>[2x]SGSMEIRVR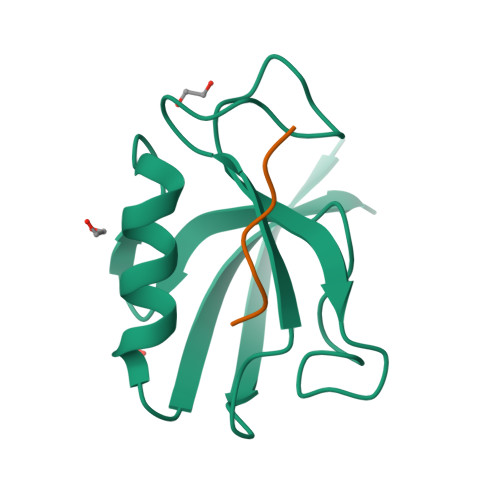VEKDPEIGFRIAGGVGGRGNPFRPDDDGIFVTRVSPEGPASKLLQPGDKIIQANGYSFINIELGQAISLLKTFQNTVELIIVREV;>[2x]YYESDWL>MSLSQEMIKKWLDEEGFLRMEVPDENARFHYVVNY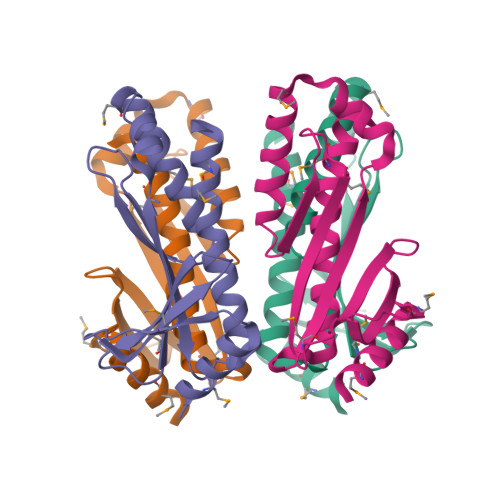PEDHVIDIIQPAGKDDMILIACATSVSPEHQAGIRALSMEKRTEFIWKVRFTLNRFGVDFQLDHPENVLNSYLVTDEIFFDGLSKDRLISSIKNVFRAKLQVMWMIQERFGEERPEHDSMYVEGHHHHHH[4x]> GPGSSLQTSDVVIHRKENEGFGFVIISSLNRPESGATITVPH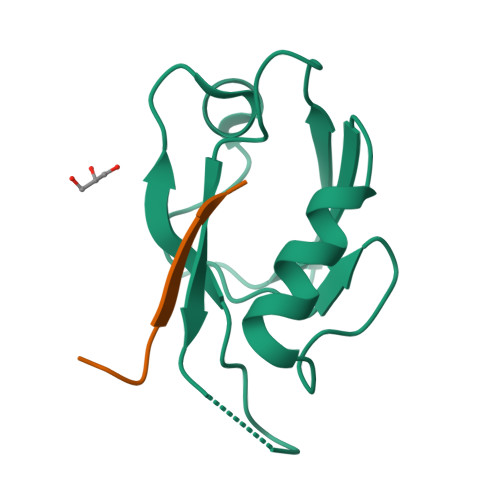KIGRIIDGSPADRCAKLKVGDRILAVNGQSIINMPHADIVKLIKDAGLSVTLRIIPQEE;> GPGSSSESTGFGEERESIL(2S,3S,4R,5S)-2-(4-amino-5H-pyrrolo[3,2-d]pyrimidin-7-yl)-5-[(propylsulfanyl)methyl]pyrrolidine-3,4-diol | C14 H21 N5 O2 S | 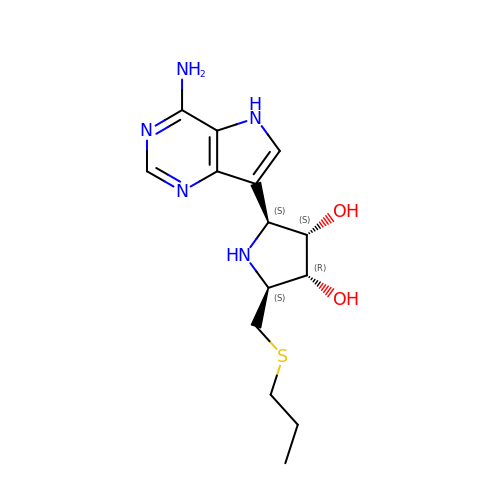SMSLFFRQRVMFGA-LGOOBZPGSA-N>[2x]MLVLGLNGNFSAADTDVVPQLGEVFFHDSAASLIRDGELVAAVEEERLNRIKKTTKFPLNAVRECLALAGARPEDVDAVGYYFPENHIDTVLNHLYTEYPRAPLRYSRELIRQRLKEGLGWDLPDEKLVYVPHHEAHAYSSYLHSGMDSALVLVLDGRGELHSGTVYRAEGTRLEKLADYPVPKSLGGLYLNATYLLGYGFGDEYKVMGLAPWGNPETYRDTFAKLYTLQDNGEYELHGNIMVPNLVSPLFYAEGFRPRRKGEPFTQAHRDFAAALQETVEKIVLHILEYWAKTSGHSRLCFGGGVAHNSSLNGLILKSGLFDEVFVHPASHDAGAGEGAAYAAAASLGTLERPGKRLLSASLGPALGGREQIRARLADWAPLIDVEFPDDAVETAAGLLAEGQVLGWAYGRSEFGPRALGHRSIVADARPEENRTRINAMVKKREGFRPFAPVVTAEAARDYFDLSGADGNHEFMSFVVPVLPERRTELGAVTHVDGTARVQVVSAESGERFHRLVRRFGELTGTPVLLNTSFNNNAEPIVQSLDDVVTSFLTTDLDVLVVEDCLVRGKASPDLGVLVPRFRPVTRLVERRTAGPDASAGAKTHEIHLDYDGGPSAKVSPELYELLGAVDGTTTLGDLAKTVGGLSDALATEVFALWEQRFLTLAPAGDIGPLADDGTRGH

Carbamoyltransferases (CTases) catalyze carbamoylation, an important modification for the bioactivity of many secondary metabolites with pharmaceutical applications. GdmN and Asm21 contribute to O-carbamoylation at the C7 (S configuration) of geldanamycin and ansamitocins, respectively. CTases in class III, which modify secondary metabolites, adopt two nucleophilic half-reactions, the formation of carbamoyl-AMP derived from ATP, CP, and Mg2+ and the subsequent transfer of the carbamoyl group from carbamoyl-AMP to the secondary metabolites. GdmN forms a face-to-face homodimer through unusual C-terminal domains, a previously unknown functional form for CTases.

Unexpectedly, structural characterization revealed the appearance of three reaction intermediates at different stages, in which two different intermediates usually resided in different subunits of a single homodimer enzyme molecule. One of the three intermediates was the natural tetrahedral intermediate carbamoyl-AMP-1, which had been predicted, but not structurally characterized, in a CTase. Structural analysis of the carbamoyl-AMP-1 tetrahedral intermediate revealed the geometric structure of a natural tetrahedral intermediate in a carbamoylation process. The carbamoyl-AMP portion remained almost in the same position, while the formation of the C-O bond between the carbamoyl group and the oxygen atom of C-7 in 1 drove a slight shift of 1 towards carbamoyl-AMP. The capture of the tetrahedral intermediate implied that this catalytic reaction proceeds in a stepwise manner rather than in a concerted process. Another intermediate was 2, which was carbamoylated, but not cyclized, with AMP located adjacent to 2. In the GdmN/AMP/2 unit, the C-7 oxygen of 2 was 2.9 Å from the lateral chain of H27. The distance between the amine of the carbamoyl group and iron ion was 3.1 Å, while the distance was 2.7 Å in the GdmN/carbamoyl-AMP/1 subunit, representing the end of the carbamoylation reaction. The structural characterization of 2 revealed the conformation of ansamycin derivatives before the formation of the C7,9-cyclic carbinolamide group, which has not been observed in other studies.> SPKYTKSVLKKGDKTNFPKKGDVVHCWYTGTLQDGTVFDTNIQTSAKKKKNAKPL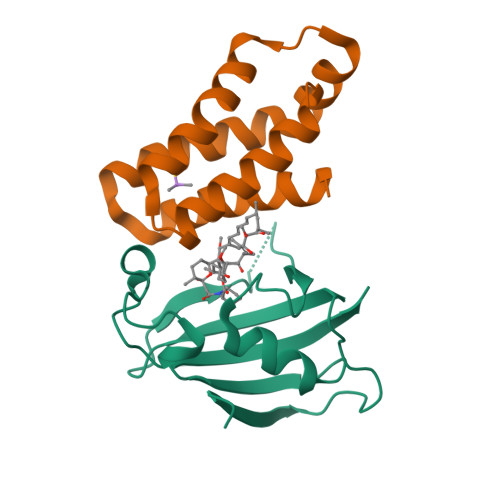SFKVGVGKVIRGWDEALLTMSKGEKARLEIEPEWAYGKKGQPDAKIPPNAKLTFEVELVDID;> SILWHEMWHEGLEEASRLYFGERNVKGMFEVLEPLHAMMERGPQTLKETSFNQAYGRDLMEAQEWCRKYMKSGNVKDLTQAWDLYYHVFRRIS> IVGGQECKDGECPWQALLINEENEGFCGGTILSEFYILT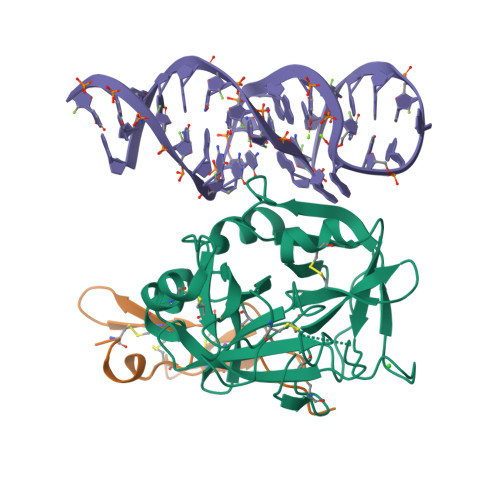AAHCLYQAKRFKVRVGDRNTEQEEGGEAVHEVEVVIKHNRFTKETYDFDIAVLRLKTPITFRMNVAPACLPERDWAESTLMTQKTGIVSGFGRTHEKGRQSTRLKMLEVPYVDRNSCKLSSSFIITQNMFCAGYDTKQEDACQGDAGGPHVTRFKDTYFVTGIVSWGEGCARKGKYGIYTKVTAFLKWIDRSMK;> LCSLDNGDCDQFCHEEQNSVVCSCARGYTLADNGKACIPTGPYPCGKQTLE> MSHHHHHHSGSMNNFNLHTPTRILFGKGAIAGLREQIPHDARVLITYGGGSVKKTGVLDQVLDALKGMDVLEFGGIEPNPAYETLMNAVKLVREQKVTFLLAVGGGSVLDGTKFIAAAANYPENIDPWHILQTGGKEIKSAIPMGCVLTLPATGSESNAGAVISRKTTGDKQAFHSAHVQPVFAVLDPVYTYTLPPRQVANGVVDAFVHTVEQYVTKPVDAKIQDRFAEGILL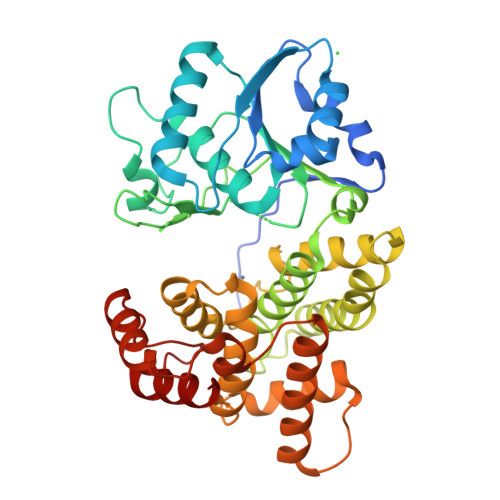TLIEDGPKALKEPENYDVRANVMWAATQAENGLIGAGVPQDWATHMLGHELTAMHGLDHAQTLAIVLPALWNEKRDTKRAKLLQYAERVWNITEGSDDERIDAAIAATRNFFEQLGVPTHLSDYGLDGSSIPALLKKLEEHGMTQLGENHDITLDVSRRIYEAAR> GPHMGLQESFGVAAEDKIFGGSGSFIPRCMEAMKGVRSMLQCMADKANARNMLQQASLVRPLDNQETLDFSRLSLVEQHECLASILHAAVQRHHATIADFQDFIKILRKWDKYDHFLIHLIPVLAAYITEFGSPEGMGDLQQARRLNDFICKGGDEDSWALPVLGAAVRAWWIAEHNGFYLDDTVQDLRGINLDEEDEQRTKQFLDALKEGAFDFILSVAADCKAQEWQDPSQLGARQWLQRKIPSLPSEPFPFSHFLQHSLMVHLEGFVDATISNLPDVLRKLRTEEDEQRQLRPNHEQDMDLERFLIIISYAYEGRPDAAMSFWEDPDSNLAGFLQWASRRASTPLVSAFCEMLRCLADNEECATAAHNFLLDEGHQASGKMKRSQSLTWSQIFKELEYFTTKVCSERPNPPQASMHRPGRPGADPAEIEPESALMLECYLRLIAKLATESEIARKRLIMDEDFNLVDTILKLSVGVIPHRLRACIFYVLKALMIRKTHEELDAMWRWVEAWMTNPFSSLPGSQGAPQRISFLGQTPGPQECMEMMFREFGTGFEQSNAFIQLLTTLLVPPEGLNSLNDSVPFPEWLGSSIRTLGIEPYVDFVFDVFANRTKDISDPSQLRILRLSCLDFVMVCLVTFNEDLIVLGHESNISIDDAMAATNLATYVRLHPFSRVMEWLFNEKVITSLINTIHQDPISLGSASPDSPLVVSILRAIQVMIKALELQETYLHLVRPEVLRYQGEAGVRRKPVANA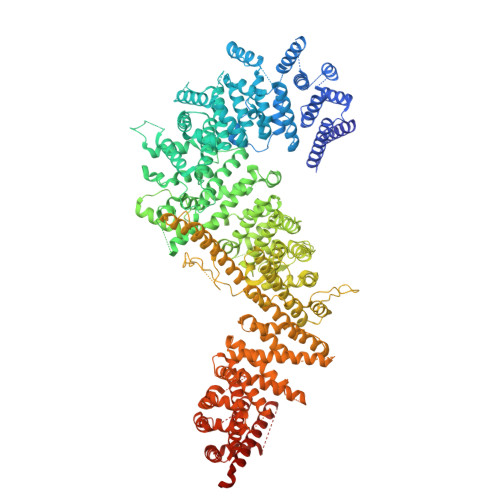AYSAFEDGILSHLSLVVDLGKYCNLGHAELTLACLKLLEKISTSSRILSAWSPDSGRLGHRNKAIVQLERNGEGETISASLSASIMATLDPALAASGENYRVKLAILDFLYACLRATPDQPTIAHQLLGFHCELSKLGIEPKGPFDMQKSLFHSLLNVLITLTVSEEEQGMRGYLVTLKYRVLRILQLLWKSPLSASLVMDELRATNFLFHMLLREVQIQPQLPWDGQLVTGCEFLLSDASLAYIDYLASRAAIFEYIGKELCSVSQNRIPSIKRQIFDALNGQIFVDEEAPLTIPSIFDFFDFINTDYKWEEIPSPHFTYLKDLDLGPCILEHKYAGVHYDIRKAQEILALKRKEYEHSQLATPEFLETVELEEKVLIEWLTVRNRANLLLTARLNLLQAWANLLLVMIESNDFKSTPKMAFLLQALQAILPTLEAFSSLKSDEAFELARVAKVLLWKLDFSQDSDAGLDREQFTVGNLIGDKLFQLFQLCLSAISQCSGTPELRSLYYSICYRYLTAVVDNDATVAATPASSTIGPTRSVTNARARTLKAITLYGDRLLNVICDDAYGSDTTCQTAAMILLNALVHTSRASSAAGVSPADVDCPIIDALNRLNFIGVLVDSLKEILNEWLAPSSTFDPSLSTNASPSLPIPASPSQQYTSAKLALLLQLCQTRQGAKYVLQANLFRALEQSGVFAADPELVEVDSESGVPRVVALERHYALLVALARVVGAAVTARGAHNIVQGRKFLTQHRGLVVHVLKKNAGIGGGVVGNSLASSINGGSTATMTRRDEILAQQALEERIEELAEAFMLLITATGFLEYESEQVPSEQPRAHTTFFH Orange Carotenoid protein (OCP) is the only known photoreceptor which uses carotenoid for its activation. It is found exclusively in cyanobacteria, where it functions to control light-harvesting of the photosynthetic machinery. In the active state, following OCPR (red state) binding to the cyanobacterial light-harvesting antenna, the keto-carotenoid dissipates excess absorbed light energy through non-photochemical quenching (NPQ), a vital process for cyanobacterial survival in turbulent waters.

The I1 dataset with 1 min illumination reveals s-trans to s-cis CAN isomerization along the C9’-C8’ single bond concerted with s-cis to s-trans isomerization along the C7’-C6’ single bond (s-BP isomerization) as the early step of activation (d and below). As a result, C8’ = C7’ changes its orientation. The refined coordinates obtained from extrapolated structure factors identify the CAN s-BP isomerization after 1 min of illumination at the experimental light intensity as a first light-activation step. In the I1 structure, no changes of coordinates are observed for W110 compared to OCPO but the Y44 sidechain undergoes a rotation by 31o. As a result of Y44 rotation by 31o in NTD in the I1 state, the distance between the hydroxyl group of Y44 and the C9’ carbon reduces by 2.0Å, redistributing charge-density around C9’-C8’. Leucine L37, which has been proposed to play an important role in OCP light-activation, does not undergo any significant movement upon illumination. We therefore conclude that the s-BP isomerization of CAN in I1 causes rearrangement of the CAN β2-ring binding pocket in the NTD, which is mediated by contact with Y44. The salt bridge rupture between R155 and E244 is already observed in I1 and increases the distance between residues E244 and R155 by 1Å. We complement this knowledge by showing that salt bridge rupture between R155 and E244, the important precursor of NTD and CTD separation, occurs in the first illumination step (I1) and is controlled by a hydrogen bonding network involving protein-bound water molecules. The I1 structure is the first example where s-BP isomerization of a carotenoid carbon chain regulates the activity or the biological function of a protein.

> MGSSHHHHHHMPFTIDSARGIFPNTLAADVVPATIARFSQLNAEDQLALIWFAYLEMGKTLTIAAPGAASMQLAENALKEIQAMGPLQQTQAMCDLANRADTPLCRTYASWSPNIKLGFWYRLGELMEQGFVAPIPAGYQLSANANAVLATIQGLESGQQITVLRNAVVDMGFTAGKDGKRIAEPVVPPQDTASRTKVSIEGVTNATVLNYMDNLNANDFDTLIELFTSDGALQPPFQRPIVGKENVLRFFREECQNLKLIPERGVTEPAEDGFTQIKVTGKVQTPWFGGNVGMNIAWRFLLNPEGKIFFVAIDLLASPKELLNFAR> MIGRKKLEEHYITIAEAKELLERRHAEGLAENPEEPMFYEARVSLEHAERFAKLKPEQARELKEKLMGLFDWINERIAAKLVDILPEDYLDIRVIFAKEEYMPTPEEAEEIIK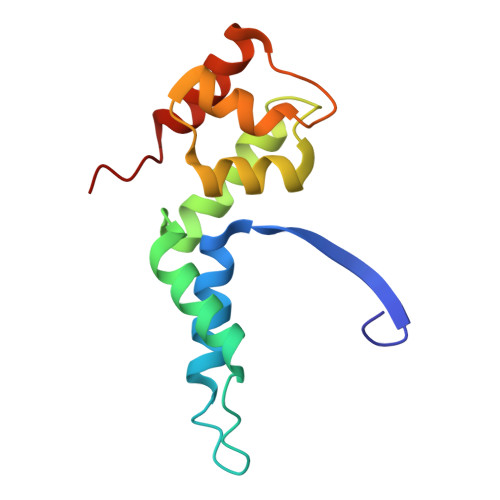VIDEYRPLE> TRDQ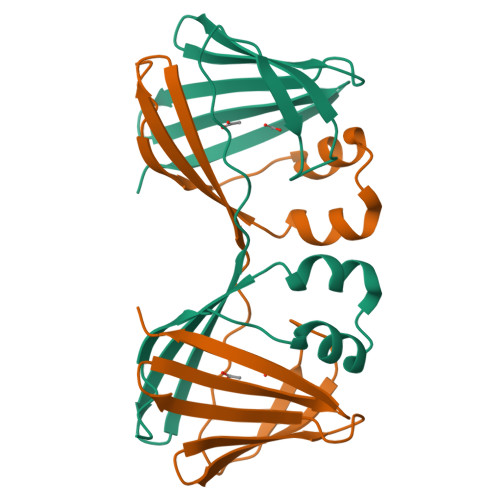NGTWEMESNENFEGYMKALDIDFATRKIAVRLTQTKVIDQDGDNFKTKTTSTFRNLDVDFTVGVEFDEYTKSLDNRHVKALVTWEGDVLVCVQKGEKENRGWKQWIEGDKLYLELTCGDQVCRQVFKKK> KDETVGVGVLSEPHARLLEIAKEEVKKQHIELRIVEFTNYV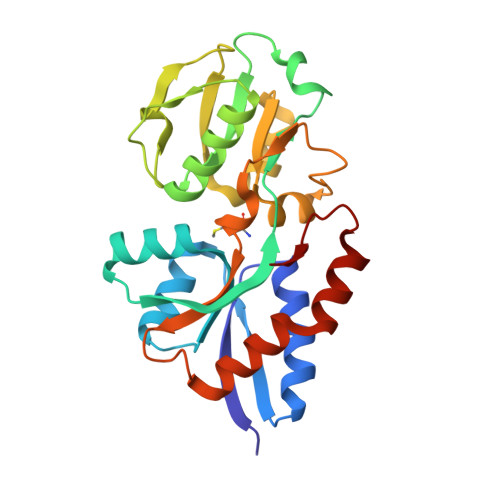ALNEAVMRGDILMNFFQHVPHMQQFNQEHNGDLVSVGNVHVEPLALYSRTYRHVSDFPAGAVIAIPNDSSNEARALRLLEAAGFIRMRAGSGLFATVEDVQQNVRNVVLQEVESALLPRVFDQVDGAVINGNYAIMAGLSARRDGLAVEPDASAYANVLVVKRGNEADARVQAVLRALCGGRVRTYLKERYKGGEVAPAL>MNPAAEAEFNILLATDSYKVTHYKQYPPNTSKVYSYFECREKKTENSKLRKVKYEETVFYGLQYILNKYLKGKVVTKEKIQEAKDVYKEHFQDDVFNEKGWNYILEKYDGHLPIEIKAVPEGFVIPRGNVLFTVENTDPECYWLTNWIETILVQSWYPITVATNSREQKKILAKYLLETSGNLDGLEYKLHDFGYRGVSSQETAGIGASAHLVNFKVTDTVAGLALIKKYYGTKDPVPGYSVPAAEHSTITAWGKDHEKDAFEHIVTQFSSVPVSVVSDSYDIYNACEKIWGEDLRHLIVSRSTQAPLIIRPDSGNPLDTVLKVLEILGKKFPVTENSKGYKLLPPYLRVIQGDGVDINTLQEIVEGMKQKMWSIENIAFGSGGGLLQKLTRDLLNCSFKCSYVVTNGLGINVFKDPVADPNKRSKKGRLSLHRTPAGNFVTLEEGKGDLEEYGQDLLHTVFKNGKVTKSYSFDEIRKNAQLNIELEAAHHLEHHHHHHHH[2x]

NAMPT functions as a homo-dimeric enzyme that catalyzes the rate limiting step in the primary salvage pathway for NAD synthesis, the transfer of a phosphoribosyl residue from 5-phosphoribosyl-1-pyrophosphate (PRPP) to nicotinamide (NAM) to produce nicotinamide mononucleotide (NMN). Crystal structures of NAMPT in numerous ligand-bound forms have been reported. These structures consistently display a NAMPT homo-dimer with two essentially identical active sites at the dimer interface. Typical NAMPT inhibitors were found to occupy the portion of active site responsible for NAM binding and a tunnel-shaped cavity extending from the NAM binding site. Furthermore, we determine the crystal structures of six NAMPT mutants in the apo form and in complex with various inhibitors and present a definitive model to explain the differential effects of the mutations on various structural classes of NAMPT inhibitors.

The crystal structures of G217 mutants revealed that they also perturbed inhibitor binding through a His191-mediated mechanism. Glycine is required for this position to allow a water molecule to bind and participate in the D219-H191-WAT-Y188 network. The addition of a Cβ atom in G217A occludes the water molecule and disrupts the hydrogen bond network. In addition, A217 pushes the H191 imidazole ring away from its normal orientation by 30°, rendering this part of the tunnel less compatible with GNE-618 binding. The conformational changes induced by G217A are amplified in the G217V mutant, where the H191 side chain is twisted 40° away from the optimal herringbone conformation. Similar to H191R, inhibitors with narrow and flexible linkers, including APO866, are less sensitive to the relatively subtle changes induced by the G217A and G217V mutations, which is also consistent with the modest drop in the biochemical potency of compounds 9-11. The RD line harboring the G217V mutation also had the D93 deletion. The D93del/G217V RD line is 500 to 4000 fold resistant suggesting that a significant increase in resistance is conferred by the G217V mutation.>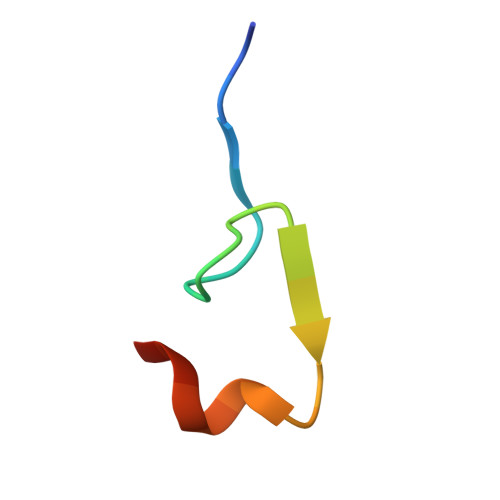 DLEVIISLGPDPTRLDAKLLDSYSTA> SKNLILDFPQPSTDYLSFRSHFQKNFVCLENCSLQERTVTGTVKVKNVSFEKKVQIRITFDSWKNYTDVDCVYMKNVYGGTDSDTFSFAIDLPPVIPTEQKIEFCISYHANGQVFWDNNDGQNYRIVHVQWKPD

Dephosphorylation of both enzymes is exerted by protein phosphatase 1 (PP1), a pleiotropic phosphatase involved in the regulation of cell growth and protein synthesis, other than glycogen metabolism. PP1 is directed to its different pathway-specific substrates by scaffold proteins; PPP1R3 are those orienting PP1 towards GYSs and PYGs. PPP1R3C (317 amino acids), also named protein targeting to glycogen (PTG), is ubiquitously expressed. PTG is composed of 317 amino acids with a structured central region, containing a carbohydrate-binding module 21 (CBM21, residues 133–261), flanked by largely disordered regions.

We determined the crystal structure of the PTG CBM21 in complex with β-cyclodextrin in two different space groups at 1.5 and 2.0 Å resolution. The domain is organized in a β-sandwich of eight antiparallel strands (β2-β9) divided into two β-sheets, with an overall immunoglobulin-like fold. On one side of the sandwich, the N-terminal region forms a short 310 helix immediately followed by an α-helix and connects to the C-terminal segment through an additional two strands short β-sheet (N-ter β1 and C-ter β10). The four chains (one in the orthorhombic crystal and three in the asymmetric unit of the monoclinic system) are identical with an average rmsd of 0.36 Å (over Cα atoms). In the PTG CBM21 crystal structure, the β-cyclodextrin molecule binds at the interface between symmetry-related copies occupying site I in one chain and site II in the other. In site I, half of the cyclodextrin molecule lies on the shallow tray generated by the β4-β5-β8-β9 sheet together with the β4-β5 and the β9-β10 loops. Major van der Waals contacts are with Arg187, Trp193, Tyr196, Cys235, and Trp246 together with H-bonds directed to Arg187, Asn248, and Asn253 side chains. At site II, the cyclic oligosaccharide inserts in between the β3-β4 and the β6-β7 loops with a close net of H-bonds connecting it to PTG residues Asn177, Phe180, Glu181, Lys182, Asp214, and Tyr203 (this last being water-mediated); additionally, extensive van der Waals contacts are present with Lys182, Tyr203 and especially Phe180 that, inserting in the cyclodextrin ring, becomes fully buried. The observed interaction at site I configures then as a crystallographic interface or as an ancillary carbohydrate-interacting site, which binding to glucose chains is cooperatively reinforced by the dominant interaction at site II; while site I shows some sequence divergence, all site II residues are conserved in PTG, GM and GL. Analogously, we measured a KD of 59 ± 5 μM with a 1:1 stoichiometry by ITC titration of PTG CBM21 with β-cyclodextrin.>[27x]MLNPNRIKDEFSVRLEDIENSINESYNLSTIGGDFAAIATDDAVFESYKDQLLEGFDAAEGEALAGMLDNTREEILMESSMGPIQPYASLSMPILVKLWARLALTEALPTQVANKPNFTVPILTPYVVDADGNKHALPESINNTPETLVGLVQIKEDIAVEGGKVTDYDLFTGLKEGKEVRKGIDRLDRKFKIVEAKWSDSFDERTSAAGFVELGSNVVKLQDNDTLVGQIKYPTNGDGEVETDTILGKVDVSSGELTLTSASGKLTDVKVKGYVASEQHTSATNVELGLTRKDVVIDTAQHIEATVPLEVIQDMKATYDIDGVARLSETMSQLSSQKVDLDIIEFLDHEYKETDAKYHFSFDVFPHSDYSAHPKDWLEGLREVIDHTTQSMKNDYKLYDVQFVIVGNPLDVRLIPNVSWTFNGGDRNADAYSNGIKINYSLGAASGTANYRIIGSDLVRQGELTIIAIPQQDNYKTFMFYPYTFNV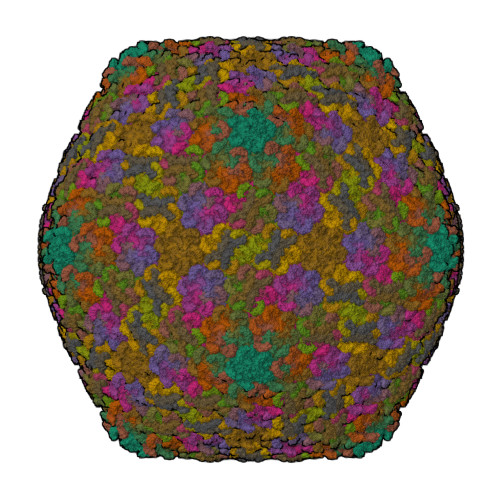VNGGGYLNTRNPNVPNMMMTRRYTVESFVPIIGRITIKNNNGSVYAR;>MATTNYFKVKLLDEKLIPFLGLGERGPRENVILSSNDLASLKQAGWTVTDVQPLPETGKIKYDRRTVYFKSEGETGKFINVPFYINPVDARDVLGLLKFDLIKLSDKSVVKTYTAKDIKSEILSLPTSDLEVNEEYELKLYFPKDASENYDIAISEGHKNLFERVKDSVFIKVKEYGKFTGRLVQLQQDINVLKESALPLDKILGYKDFDTKEVTPVAKENLLQLLSVNVSDESYARYQADKNRLLFFSKTGEILVKVIERSIQDNIVNFNIRILDEETIQNEIDKKIEYSVYDPKDGKFESINQTKSITVTPETVNIEAEQTQKLEVTTEPEGRKVSFELKDGSEFASVDNNGNITGISEGTANVTVKSDDVSKNVEVNVSRLKTKSLTVTPEEVNIDAESTQQLDVKIQPSTNSVSYSITEGSEYASVNNSGLVTAKAAGTAKVKVTSDSVSKDVSVTISTSQVEETPEETTTE[4x]2-(5-phenyl-4-{(R)-phenyl[2-(piperidin-1-yl)ethoxy]methyl}-1H-pyrazol-1-yl)pyridine-4-carboxylic acid | 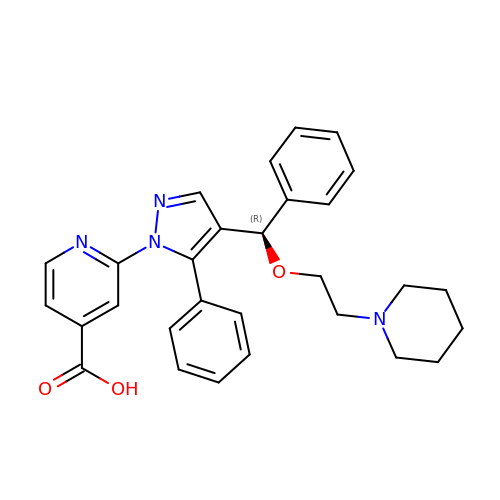C29 H30 N4 O3 | HAJRSCRWEDXEKU-MUUNZHRXSA-N> MAKATTSVNYACNLDKRLPELPEGANRAQILESTWSTEFKVYDSFGEAHELQIDFARVPGEVNAWRATVNVDPTNADATATRVGIGTTDGV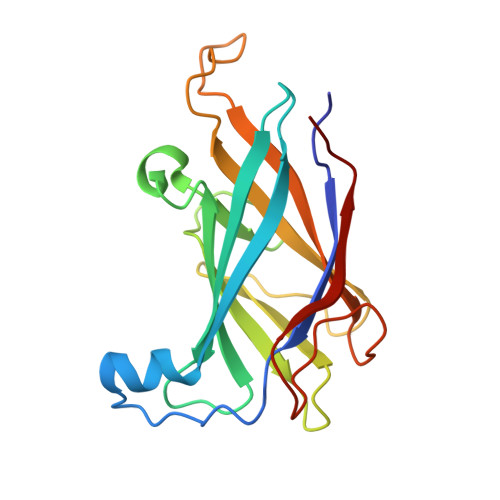QNSFIVRFDNNGHLASVTDTAGNVTSPAGQVLVQISYNVVGANPDEAGAPTRHTFDVNLGEIGTSKNTITQFSDKSTTAAYEQDGYT>MHHHHHHLVPRGSHMSVVGTPKSAEQIQQEWDTNPRWKDVTRTYSAEDVVALQGSVVEEHTLARRGAEVLWEQLHDLEWVNALGALTGNMAVQQVRAGLKAIYLSGWQVAGDANLSGHTYPDQSLYPANSVPQVVRRINNALQRADQIAKIEGDTSVENWLAPIVADGEAGFGGALNVYELQKALIAAGVAGSHWEDQLASEKKXGHLGGKVLIPTQQHIRTLTSARLAADVADVPTVVIARTDAEAATLITSDVDERDQPFITGERTREGFYRTKNGIEPCIARAKAYAPFADLIWMETGTPDLEAARQFSEAVKAEYPDQMLAYNCSPSFNWKKHLDDATIAKFQKELAAMGFKFQFITLAGFHALNYSMFDLAYGYAQNQMSAYVELQEREFAAEERGYTATKHQREVGAGYFDRIATTVDPN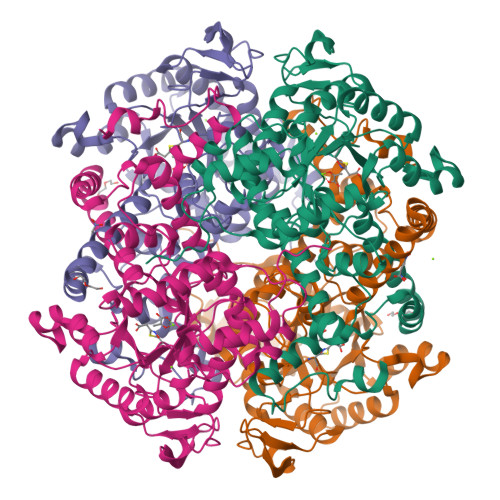SSTTALTGSTEEGQFH[8x]>MSDKIIHLTDDSFDTDVLKADGAILVDFWAEWCGPCKMIAPIL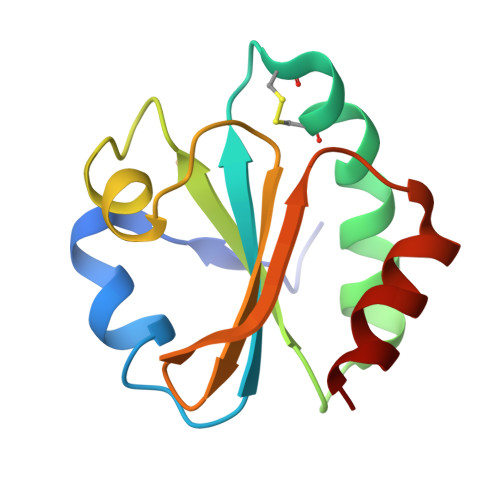DEIADEYQGKLTVAKLNIDQNPGTAPKYGIRGIPTLLLFKNGEVAATKVGALSKGQLKEFLDANAA[7x]>MWYTGTGDKGKTKVPSVGEVWKDSEIVKALGDLDELNSVLGVVSSLYPELSEVIQKLQNDIFSISSEIAGFDMNFSDEKVKGIEELITNYSKELEPLRNFVLPGGHIASSFLHLARAVCRRAER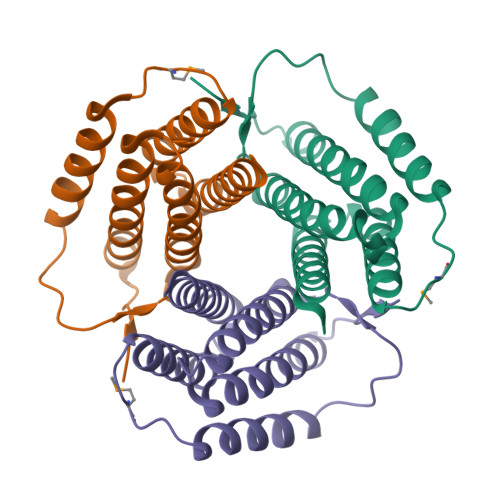SVVTLLKESKAKEVHAKYLNRLSSLLFVLALVVNKRTNNPNVIWRGKD[3x]> MGRVE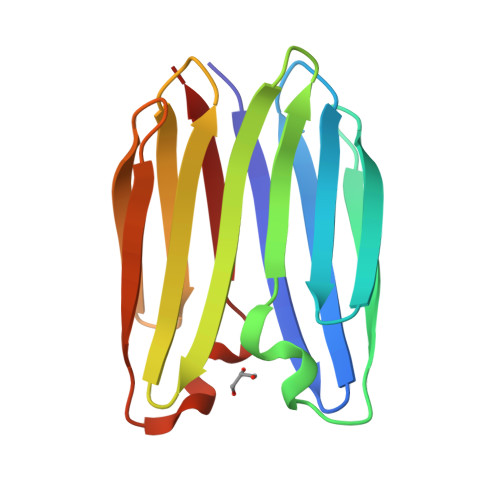VRVEFEGDKMRVRLRNDSSTPVEVHIKVGDEKRTVTVNPGEEVEVTFSANDPHKFNRPQFTIEWGGGGRVEVRVEFEGDKMRVRLRNDSSTPVEVHIKVGDEKRTVTVNPGEEVEVTFSANDPHKFNRPQFTIEWG> MLRRQCVVLSYQRGSWAPGSKHQKHMSLNPTMYLYRFAGPHGPGPYVMKYWWTLGCFPTGIERPFRLPEFLASYQQQHVPIEVEEWLQCFVKNPYEELKDATSSLLKCLEEVPIRENTRGYRSIESGVSSFAAPLAQFERQLNVRVPSLAVRAALGSPALRERLKDDLFEYNESLSACGSTPHRRLARLAFDEPLTLPGGINNSDDSENLRGQISVPMSEAIGSYASPNPSTSDDEKKLIRLLTTFSEGCTLKEDYESAFSLLSSSLGFSHDDNTDGVVHSNASAAAILGGLYKEAEFHGRQAALLEPQAMSSRKSGGRGYVLWATATAYQEDFDRASRIVEKGLEVFPDNADLKSIQEKLAGAVPAASSASPLCTRMVRSKGQQARALLHGSGRSFDNEFDWVVFKNKLYPSKM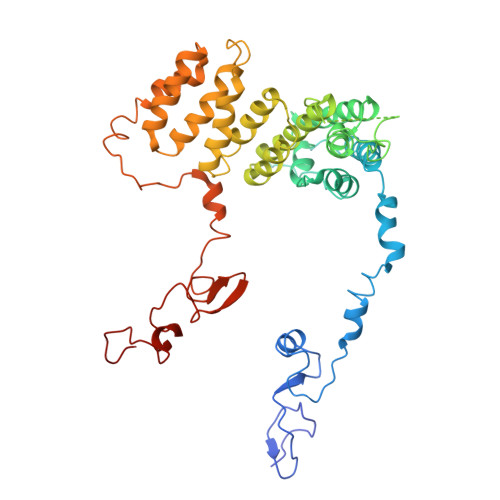NPSSNEMGSVFRRVGDFGGHISTSRSLEPL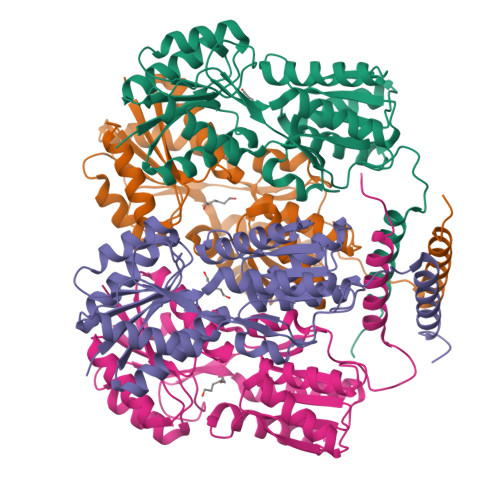>[4x]MKPVTLYDVAEYAGVSYQTVSRVVNQASHVSAKTREKVEAAMAELNYIPNRVAQQLAGKQSLLIGVATSSLALHAPSQIVAAIKSRADQLGASVVVSMVERSGVEACKAAVHNLLAQRVSGLIINYPLDDQDAIAVEAACTNVPALFLDVSDQTPINSIIFSHEDGTRLGVEHLVALGHQQIALLAGPLSSVSARLRLAGWHKYLTRNQIQPIAEREGDWSAMSGFQQTMQMLNEGIVPTAMLVANDQMALGAMRAITESGLRVGADISVVGYDDTEDSSCYIPPLTTIKQDFRLLGQTSVDRLLQLSQGQAVKGNQLLPVSLVKRKTTLAPNTQTASPRALADSLMQLARQVSRLESGQ>MTIEELKTRLHTEQSVCKTETGIDQQKANDVIEGNIDVEDKKVQLYCECILKNFNILDKNNVFKPQGIKAVMELLIDENS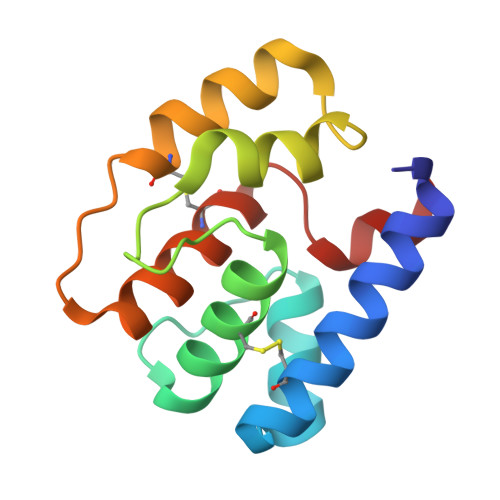VKQLVSDCSTISEENPHLKASKLVQCVSKYKTMKSVDFL[2x]> HISLNPDLANEDEVNSCDYWRHCAVDGFLCSCCGGTTTTCPPGSTPSPISWIGTCHNPHDGKDYLISYHDCCGKTACGRCQCNTQTRERPGYEFFLHNDVN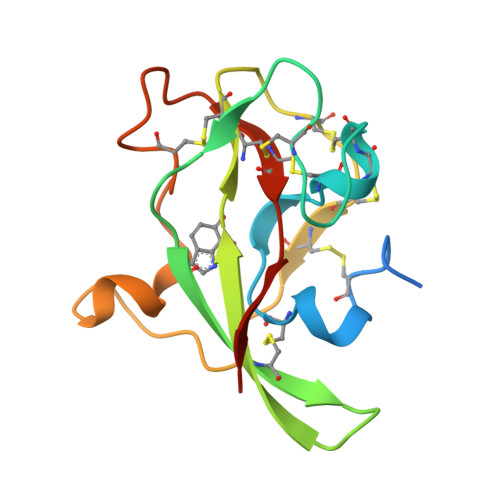WCMANENSTFHCTTSVLVGLAKN> MTLATKVFKLSFKTPVHFGKKRLSDGEMTITADTLFSALFIETLQLGKDTDWLLNDLIISDTFPYENELYYLPKPLIKIDSKEEDNHKAFKKLKYVPVHHYNQYLNGELSAEDATDLNDIFNIGYFSLQTKVSLIAQETDSSADSEPYSVGTFTFEPEAGLYFIAKGSEETLDHLNNIMTALQYSGLGGKRNAGYGQFEYEIINNQQLSKLLNQNGKHSILLSTAMAKKEEIESALKEARYILTKRSGFVQSTNYSEMLVKKSDFYSFSSGSVFKNIFNGDIFNVGHNGKHPVYRYAKPLWLEV;>MILAKTKSGKTIDLTFAHEVVKSNVKNVKDRKGKEKQVLFNGLTTSKLRNLMEQVNRLYTIAFNSNEDQLNEEFIDELEYLKIKFYYEAGREKSVDEFLKKTLMFPIIDRVIKKESKKFFLDYCKYFEALVAYAKYYQKED[2x];>[3x]MYSKIKISGTIEVVTGLHIGGGGESSMIGAIDSPVVRDLQTKLPIIPGSSIKGKMRNLLAKHFGLKMKQESHNQDDERVLRLFGSSEKGNIQRARLQISDAFFSEKTKEHFAQNDIAYTETKFENTINRLTAVANPRQIERVTRGSEFDFVFIYNVDEESQVEDDFENIEKAIHLLENDYLGGGGTRGNGRIQFKDTNIETVVGEYDSTNLKIK;> MTIKNYEVVIKTLGPIHIGSGQVMKKQDYIYDFYNSKVYMINGNKLVKFLKRKNLLYTYQNFLRYPPKNPRENGLKDYLDAQNVKQSEWEAFVSYSEKVNQGKKYGNTRPKPLNDLHLMVRDGQNKVYLPGSSIKGAIKTTLVSKYNNEKNKDIYSKIKVSDSKPIDESNLAIYQKIDINKSEKSMPLYRECIDVNTEIKFKLTIEDEIYSINEIEQSIQDFYKNYYDKWLVGFKETKGGRRFALEGGIPDVLNQNILFLGAGTGFVSKTTHYQLKNRKQAKQDSFEILTKKFRGTYGKMKEIPSNVPVALKGTTNQS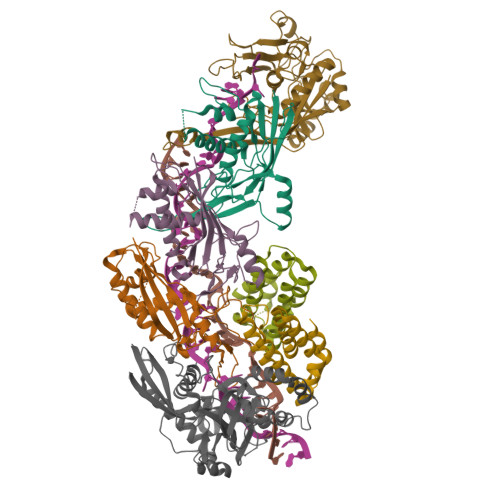RHTSYQQGMCKVSFQELNNEVL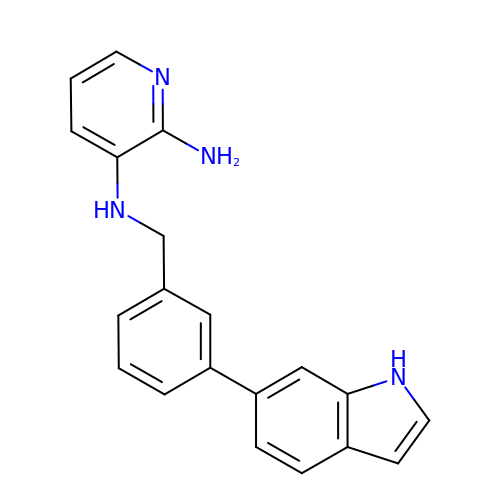N~3~-[3-(1H-INDOL-6-YL)BENZYL]PYRIDINE-2,3-DIAMINE | C20 H18 N4 | LPQUIIHPUGDHJK-UHFFFAOYSA-N>[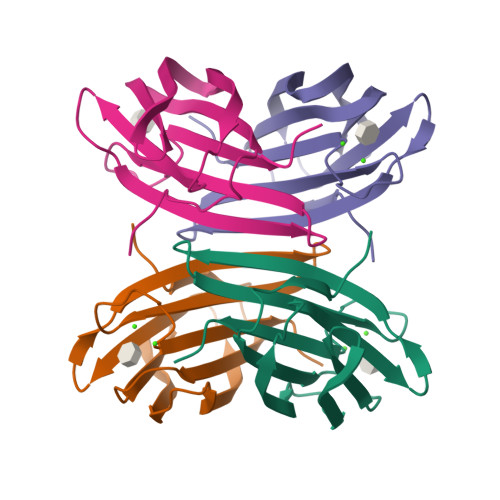4x]MATQGVFTLPANTRFGVTAFANSAGTQTVNVLVNNETAATFSGQSTNNAVIGTQVLNSGSSGKVQVQVSVNGRPSDLVSAQVILTNELNFALVGSEDGTDNDYNDAVVVINWPLG5-chloranyl-2,3-dihydroindole-1-carboxamide | C9 H9 Cl 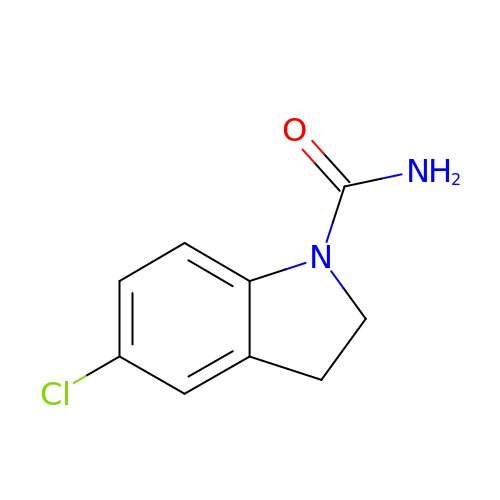N2 O | BOMYLDVQOSGKAD-UHFFFAOYSA-N alpha-D-threo-hexo-2,5-diulo-2,6-pyranosyl fluoride | 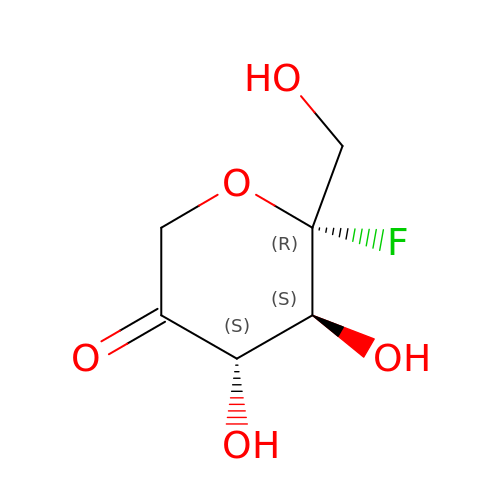C6 H9 F O5 | VCJAHEOIRFFLTQ-SRQIZXRXSA-N> GSGSRPHLAGTHTSLRLPQEGKGTCILVGGHEITSGLEVISSLRAIHGLQVEVCPLNGCDYIVSNRMVVERRSQSEMLNSVNKNKFIEQIQHLQSMFERICVIVEKDREKTGDTSRMFRRTKSYDSLLTTLIGAGIRILFSSCQEETADLLKELSLVEQRKNVGIHVPTVVNSNKSEALQFYLSIPNISYITALNMCHQFSSVKRMANSSLQEISMYAQVTHQKAEEIYRYIHYVFDIQMLPNDLNQDRLKSDI;> GSHMEKNPPDDTGPVHVPLGHIVANEKWRGSQLAEEMQGKIKLIFEDGLTPDFYLSNRCCILYVTEADLVAGNGYRKRLVRVRNSNNLKGIVV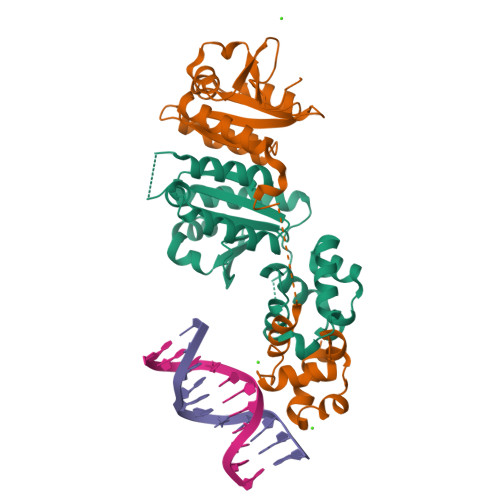VEKTRMSEQYFPALQKFTVLDLGMVLLPVASQMEASCLVIQLVQEQTKEPSKNPLLGKKRALLLSEPSLLRTVQQIPGVGKVKAPLLLQKFPSIQQLSNASIGELEQVVGQAVAQQIHAFFTQP> QCDNFPQMLRDLRDAFSRVKTFFQTKDEVDNLLLKESLLEDFKGYLGCQALSEMIQFYLEEVMPQAENQDPEAKDHVNSLGENLKT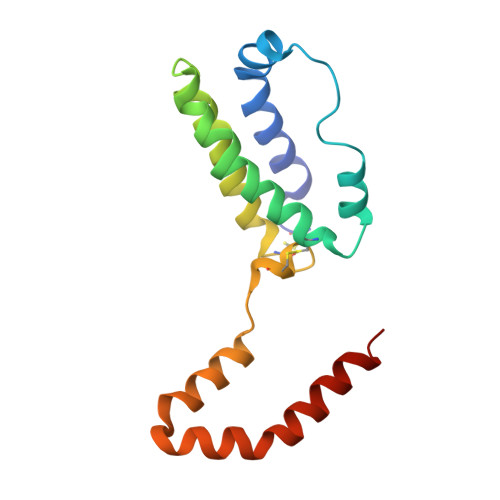LRLRLRRCHRFLPCENKSKAVEQIKNAFNKLQEKGIYKAMSEFDIFINYIEAYMTIKAR> HHHHHHMGRTVVVLGGGISGLAASYHLSRAPCPPKVVLVESSERLGGWIRSVRGPNGAIFELGPQGIRPAGALGARTLLLVSELGLDSEVLPVRGDHPAAQNRFLYVGGALHALPTGLRGLLRPSPPFSKPLFWAGLRELTKPRGKEPDETVHSFAQRRLGPEVASLAMDSLCRGVFAGNSRELSIRSCFPSLFQAEQTHRSILLGLLLGAGRTPQPDSALIRQALAERWSQWSLRGGLEMLPQALETHLTS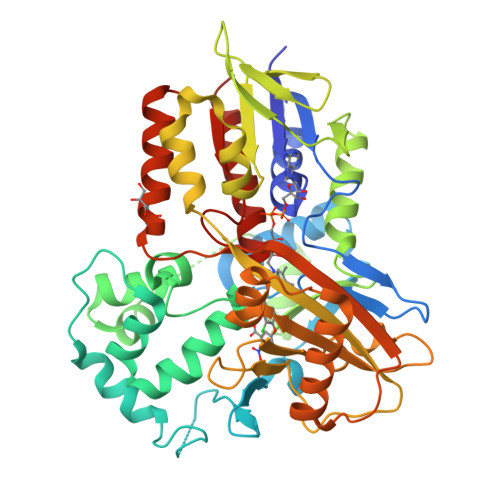RGVSVLRGQPVCGLSLQAEGRWKVSLRDSSLEADHVISAIPASVLSELLPAEAAPLARALSAITAVSVAVVNLQYQGAHLPVQGFGHLVPSSEDPGVLGIVYDSVAFPEQDGSPPGLRVTVMLGGSWLQTLEASGCVLSQELFQQRAQEAAATQLGLKEMPSHCLVHLHKNCIPQYTLGHWQKLESARQFLTAHRLPLTLAGASYEGVAVNDCIESGRQAAVSVLGTEPNS(3R,4R)-4-[4-cyclopropyl-5-[3-(2-methylpropyl)cyclobutyl]-1,2,4-triazol-3-yl]-N-(2,4-dimethylphenyl)-1-ethanoyl-pyrrolidine-3-carboxamide | C28 H39 N5 O2 | 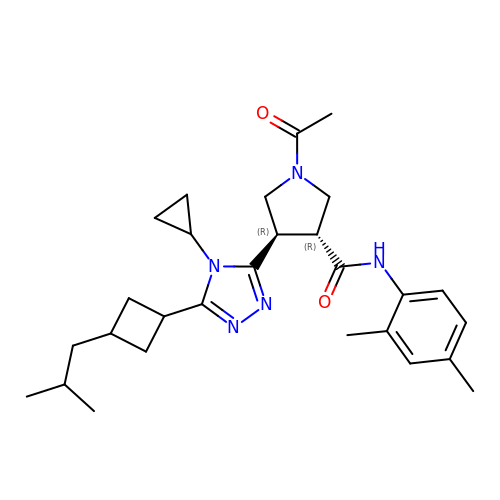NRAQMBSBKYAKMR-DVKRWUGUSA-N> ASMTIVDCGPPDDLPSGRVEYITGPGVTTYKAVIQYSCEETFYTMKVNDGKYVCDADGFWTSSKGEKSLPVCEPVCGLSARTTGGR;> IYGGQKAKPGDFPWQVLILGGTTAAGALLYDNWVLTAAHAVYEQKHDASALDIRMGTLKRLSPHYTQAWSEAVFIHEGYTHDAGFDNDIALIKLNNKVVINSNITPICLPRKEAESFMRTDDIGTASGWGLTQ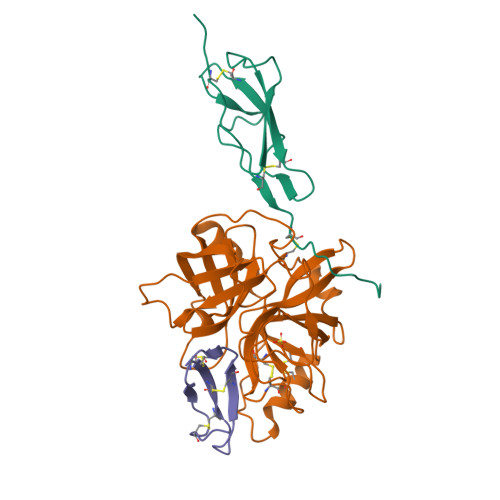RGFLARNLMYVDIPIVDHQKCTAAYEKPPYPRGSVTANMLCAGLESGGKDSCRGDSGGALVFLDSETERWFVGGIVSWGSMNCGEAGQYGVYTKVINYIPWIENIISDF;> GSGEVTCEPGTTFKDKCNTCRCGSDGKSAVCTKLWCNQ2-[2,5-bis(fluoranyl)phenyl]pyrrolidine | C10 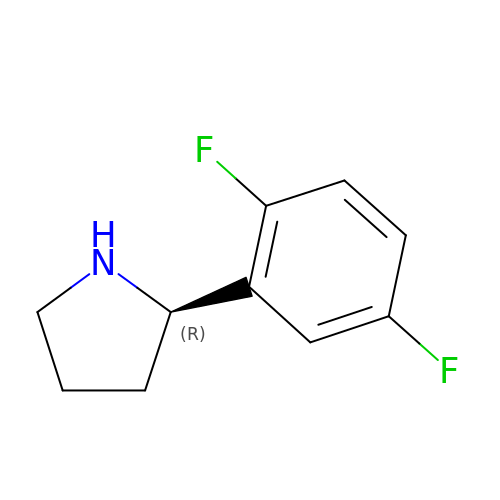H11 F2 N | NCXSNNVYILYEBC-SNVBAGLBSA-N>[2x]GSHMYRHELGMNYNFIRPDLIVGSCLQTPEDVDKLRKIGVKTIFCLQQDPDLE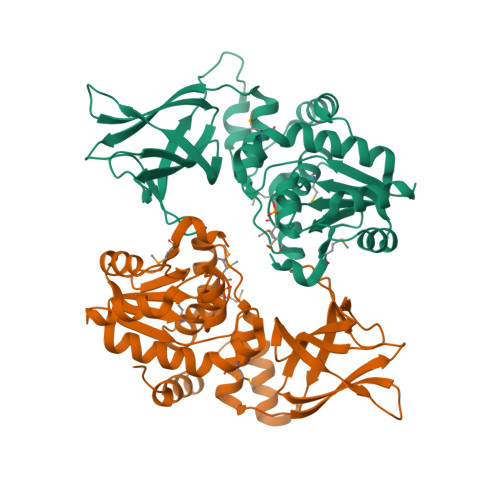YFGVDISSIQAYAKKYSDIQHIRCEIRDFDAFDLRMRLPAVVGTLYKAVKRNGGVTYVHSTAGMGRAPAVALTYMFWVQGYKLMEAHKLLMSKRSCFPKLDAIRNATIDILTGLKRKTVTLTLKDKGFSRVEISGLDIGWGQRIPLTLGKGTGFWILKRELPEGQFEYKYIIDGEWTHNEAEPFIGPNKDGHTNNYAKVVDDPTSVDGTTRERLSSEDPELLEEERSKLIQFLETCSEAEV> GSPELRQEHQQLAQEFQQLLQEIQQLGRELLKGELQGIKQLREASEKARNPEKKSVLQKILEDEEKHIELLETLQQTGQEAQQLLQELQQTGQELWQLGGSGGPELRQKHQQLAQKIQQLLQKHQQLGAKILEDEEKHIELLETILGGSGGDELRELLKGELQGIKQYRELQQLGQKAQQLVQKLQQTGQKLWQLG

Recently, we described the multi-step electron-transfer activity of a designed reaction center maquette protein (the RC maquette), which can assemble metal ions, tyrosine, a Zn tetrapyrrole, and heme into an electron-transport chain. The RC maquette integrates a Co or Fe porphyrin electron acceptor (A-site), a Zn porphyrin pigment (P-site), and an electron donating di-metal center and tyrosine (D-site) for photoactive charge separation. The RC maquette is composed of a cyt. b/b 6-like pigment/electron acceptor (P/A) module and a bacterioferritin-like electron donor (D) module. To fuse the electron donating di-metal/Tyr portion of the RC maquette to the pigment/electron acceptor domain, we joined the corresponding helices together to make an extended 7-nm long antiparallel four-helix bundle.

A complete understanding of cofactor binding requires consideration of the apo-state structure and its transition to the holo-state. The heme-bound and heme-free structures align with a Cα RMSD of 1.2 Å when inter-helical loops are not included in the alignment. The heme-free structure was obtained using a crystallization condition that included a large excess of CdCl2. Several Cd(II) ions are resolved in the structure, one of which effectively takes the place of the heme by coordinating the two A-site His residues as well as two water molecules. An additional water molecule in the A-site is hydrogen bonded to Gln111, and the side chains of Trp, Gln, and Leu residues adopt rotamers that would clash with the heme cofactor were it present. Only one of the two His-Thr pairs in the A-site forms a hydrogen bond in the heme-free structure, whereas both hydrogen bonds form when heme is present. These structural differences suggest that the cofactor binding site is only partially pre-organized prior to heme binding. Given that the a/d core of the RC maquette near the A-site includes two Gly, two His, and two Arg residues, all of which are likely to be strongly destabilizing in the apo-state, perhaps it is unsurprising that crystallization attempts without a stabilizing A-site ligand were unsuccessful. In the RC maquette, the high heme affinity and mostly folded but flexible apo-state indicate that the partial fold option has been applied successfully in a de novo-designed heme-binding protein.(S)-1-[2'-DEOXY-3',5'-O-(1-PHOSPHONO)BENZYLIDENE-B-D-THREO-PENTOFURANOSYL]THYMINE 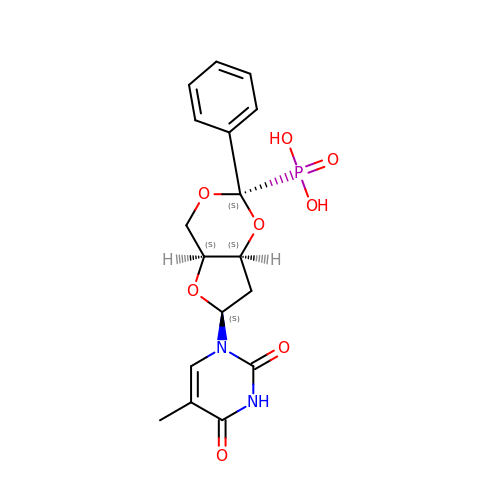| C17 H19 N2 O8 P | WTZFKHNHHRPQOU-WSMBLCCSSA-N> GSQMAISGGFIRRVTNDARENEMDE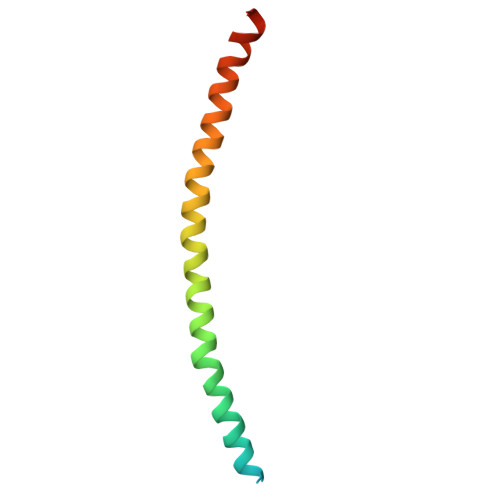NLEQVSGIIGNLRHMALDMGNEIDTQNRQIDRIMEKADSNKTRIDEANQRATKMLGSG>GKAFDDGAFTGIREINLSYNKETAIGDFQVVYDLNGSPYVGQNHKSFITGFTPVKISLDFPSEYIMEVSGYTGNVSGYVVVRSLTFKTNKKTYGPYGVTSGTPFNLPIENGLIVGFKGSIGYWLDYFSMYL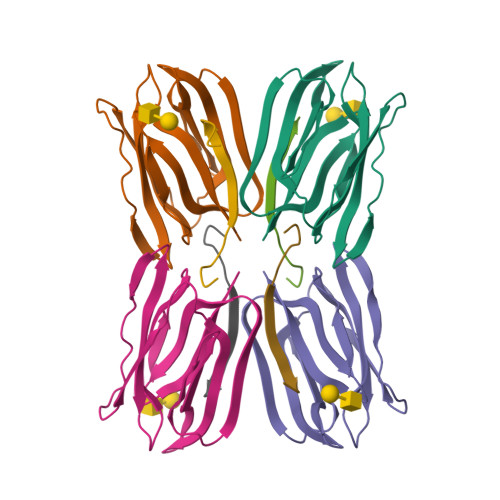SL[4x];>[4x]SGISQTVIVGPWGAKSA UBR4 is a 574 kDa E3 ligase (E3) of the N-degron pathway with roles in neurodevelopment, age-associated muscular atrophy and cancer. Here we identify and characterize a distinct E3 module within human UBR4 consisting of a ‘hemiRING’ zinc finger, a helical-rich UBR zinc-finger interacting (UZI) subdomain, and an N-terminal region that can serve as an affinity factor for the E2 conjugating enzyme (E2). Via an allosteric mechanism, the UZI subdomain modestly activates the Ub-loaded E2 (E2∼Ub).

Diffraction data were collected, and a 1.8 Å structure was solved using the anomalous signal from a single zinc ion present in the protein. Residues 4,730–4,830 of UBR4xtal were not resolved, so a model could only be built for residues 4,831–5,183. Our structure is composed of two apparent subdomains that constitute a larger fold. The N-terminal subdomain comprises residues 4,835–4,948 and is followed by the second subdomain containing 11 α-helices that run to the native UBR4 C-terminus. As such, we consider this subdomain a novel fold and refer to it as the UBR zinc-finger interacting (UZI) region. Our experimental structure confirms the structural role of conserved residues Cys4838, Cys4841, Cys4890 and His4887 as zinc coordinating ligands. Although not evident from primary sequence, the zinc finger has partial structural homology with canonical RING domains (DALI Z-score range 2.0–5.8). However, residues essential for coordinating the second zinc ion (referred to hereon as the distal Zn2+ site) are conspicuously absent. Substituting for the second zinc ion are four residues that form hydrogen bonds, and are probably required for stabilizing the cross-brace architecture of the zinc finger subdomain. However, the SP-RING maintains the distal Zn2+ site, rather than the proximal site, and lacks the extended βAB sheet. Thus, to our knowledge, the UBR4 zinc finger has unprecedented RING-related architecture, and we refer to it as the hemiRING.

> GPLGSAIQHPGTQVLIGTDSIPNLHKLEQVSSDEGIGTLAENLLEALREHPDVNKKIDAARRETRAEKKRMAMAMRQKALGTLGMTTNEKGQVVTKTALLKQMEELIEEPGLTCCICREGYKFQPTKVLGIYTFTKRVALEELENKPRKQQGYSTVSHFNIVHYDCHLAAVRLARGREEWESAALQNANTKCNGLLPVWGPHVPESAFATCLARHNTYLQECTGQREPTYQLNIHDIKLLFLRFAMEQSFSADTGGGGRESNIHLIPYIIHTVLYVLNTTRATSREEKNLQGFLEQPKEKWVESAFEVDGPYYFTVLALHILPPEQWRATRVEILRRLLVTSQARAVAPGGATRLTDKAVKDYSAYRSSLLFWALVDLIYNMFKKVPTSNTEGGWSCSLAEYIRHNDMPIYEAADKALKTFQEEFMPVETFSEFLDVAGLLSEITDPESFLKDLLNSVP N-{4-[2-([1,3]thiazolo[5,4-c]pyridin-2-yl)phenoxy]phenyl}acetamide | C20 H15 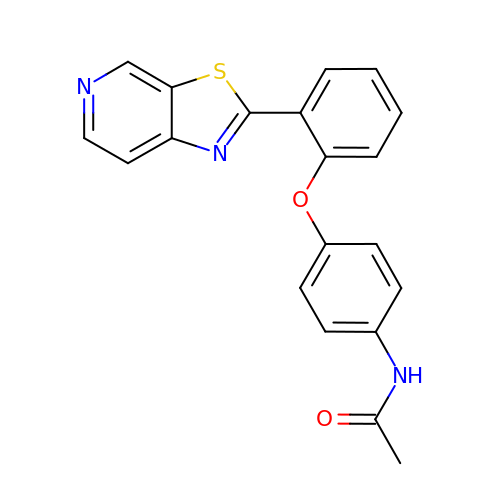N3 O2 S | OPOGWEXFOKBMCJ-UHFFFAOYSA-N> MIVLFVDFDYFAAQVEEVLNPSLKGKPVVVCVFSGRFEDSGAVATANYEARKFGVKAGIPIVEAKKILPNAVYLPMRKEVYQQVSSRIMNLLREYSEKIEIASIDEAYLDISDKVRDYREAYNLGLEIKNKILEKEKITVTVGISKNKVFAKIAADMAKPNGIKVID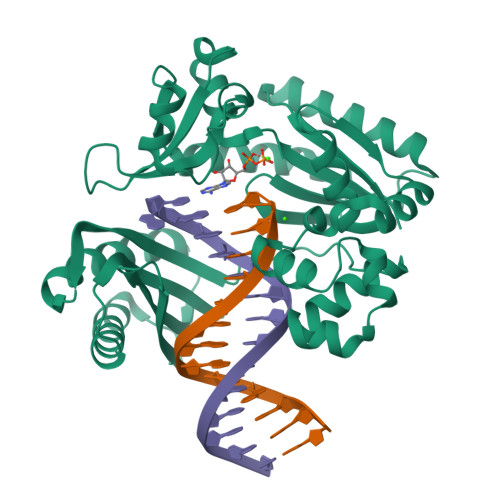DEEVKRLIRELDIADVPGIGNITAEKLKKLGINKLVDTLSIEFDKLKGMIGEAKAKYLISLARDEYNEPIRTRVRKSIGRIVTMKRNSRNLEEIKPYLFRAIEESYYKLDKRIPKAIHVVAVTEDLDIVSRGRTFPHGISKETAYSESVKLLQKILEEDERKIRRIGVRFSKFI> GKVVI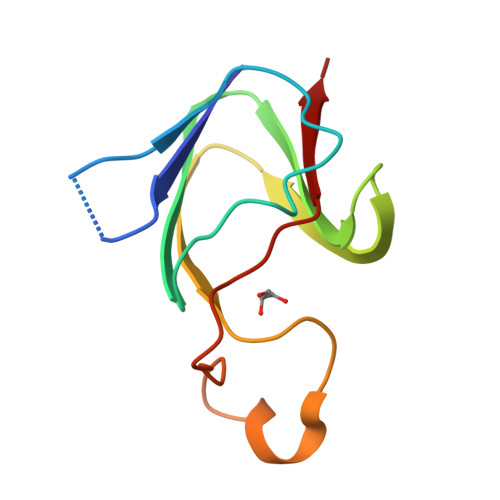YSEPDVSEKCIEVFSDIQDCSSWSLSPVILIKVVRGCWILYEQPNFEGHSIPLEEGELELSGLWGIEDILERHEEAESDKPVVIGSIRHVV(2R,4S,5S,7S)-5-AMINO-N-BUTYL-4-HYDROXY-7-[4-METHOXY-3-(3-METHOXYPROPOXY)BENZYL]-2,8-DIMETHYLNONANAMIDE | C27 H48 N2 O5 | 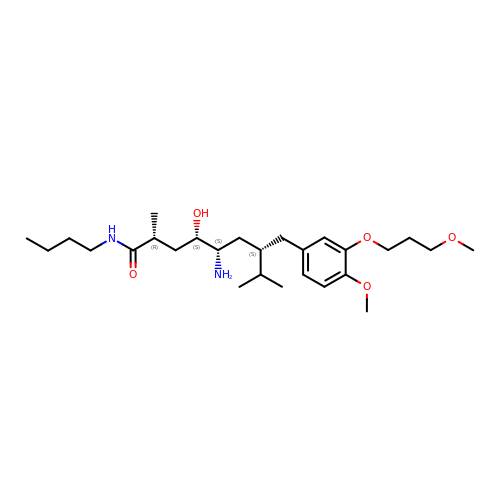HMXUWQWZWZLSAO-KAMZKSLDSA-N>[2x]MSGNGNAAATAEENSPKMRVIRVGTRKSQLARIQTDSVVATLKASYPGLQFEIIAMSTTGDKILDTALSKIGEKSLFTKELEHALEKNEVDLVVHSLKDLPTVLPPGFTIGAICKRENPHDAVVFHPKFVGKTLETLPEKSVVGTSSLRRAAQLQRKFPHLEFRSIQ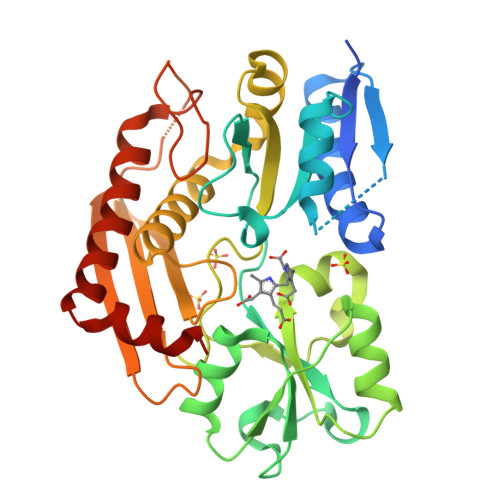GNLNTRLRKLDEQQEFSAIILATAGLQRMGWHNRVGQILHPEECMYAVGQGALGVEVRAKDQDILDLVGVLHDPETLLRCIAERAFLRHLEGGCSVPVAVHTAMKDGQLYLTGGVWSLDGSDSIQETMQATIHVPAQHEDGPEDDPQLVGITARNIPRGPQLAAQNLGISLANLLLSKGAKNILDVARQLNDAH> GVPTYLLPGSGQFLTTDDHSSAPVLPCFNPTPEMHIPGQVRNMLEVIQVESMMEINNTENAVGMQRLKVDISVLT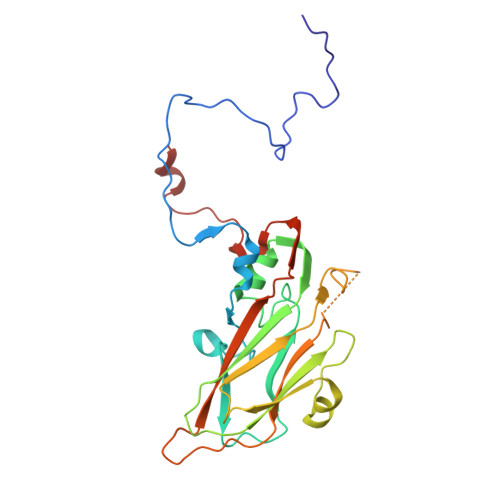DVDQLLFNIPLDIQLDGPLRNTLVGNISRYYTHWSGSLEMTFMFCGSFMATGKLILCYTPPGGSCPTTRETAMLGTHIVWDFGLQSSVTLVIPWISGSHYRMFNNDAKSTNANVGYVTCFMQTNLIVPSESSNTCSLIGFVAAKDDFSLRLMRDSPDIGQLEHLHEAEAAYQ>MRGETLKLKKDKRREAIRQQIDSNPFITDHELSDLFQVSIQTIRLDRTYLNIPELRKRIKLVAEKNYDQISSIEEQEFIGDLIQVNPNVKAQSILDITSDSVFHKTGIARGHVLFAQANSLCVALIKQPTVLTHESSIQFIEKVKLNDTVRAEARVVNQTAKHYYVEVKSYVKHTLVFKGNFKMF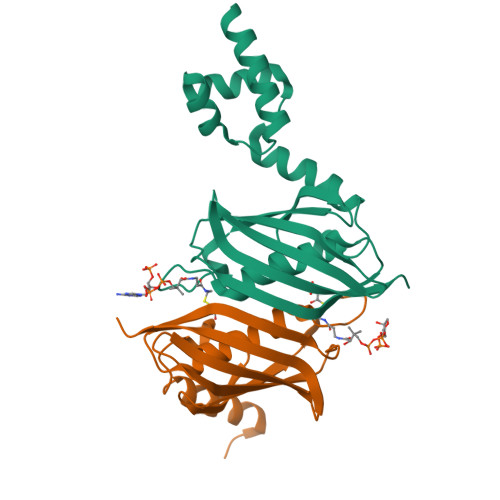YDKRG[2x]The enzyme responsible for the core function of heterotrophic nitrification is pyruvic oxime dioxygenase (POD). POD is a non-heme, Fe(II)-dependent enzyme that catalyzes the dioxygenation of pyruvic oxime to produce pyruvate and nitrite. Bacteria of the genera Alcaligenes and Pseudomonas are known to perform heterotrophic nitrification, which produces nitrite from ammonia using pyruvate oxime (PO) as an intermediate metabolite. PODs have additional sequences at the N-terminus consisting of 20–30 amino acid residues that are not present in class II aldolases, corresponding to the disordered region of AfPOD in its crystal structure.

Since an AfPODdN18 variant lacking the N-terminal 18 amino acid residues showed no POD activity, the N-terminal region should play an important role in the POD activity. The crystal structures of AfPOD and AfPODdN18 were determined at resolutions of 1.76 and 1.55 Å, respectively. The structure of AfPODdN18 crystallized in the coexistence of manganese was determined as a tetramer containing 918 amino acid residues, 682 water molecules, and 4 metal ions. The N-terminal regions (Met19-Arg28) and C-terminal regions (Lys259-Arg261) of each subunit showed no apparent electron densities. The overall structure of AfPODdN18 is nearly identical to the AfPOD with a Cα root mean square deviation (RMSD) of 0.3 Å (845 Cα atoms). The anomalous difference Fourier maps suggested that the electron density near the His triad in the AfPODdN18 is not a manganese ion. Nickel or cobalt ions may have been bound to the His triad, rather than manganese, during overexpression or purification. The dN18 variant of AfPOD completely lost its enzymatic activity, indicating that the POD-specific N-terminal extension of about 30 amino acid residues, which is not present in other class II aldolases, is essential for catalytic activity.

>[4x]MATHLQQVQRDTRETMAFACRILAMTEQEAGLAGQISVRSERPGAYWTLRFGLGFDEATPEDFIEVDRDLNTLSGEGMANPATRFHLWVYEARPDVNSIIHTHSPWATVLATARQPLVISQMDMTPLHNDCAFLGEWPGVPIADQEGVIISKALGDKRAIILAHHGYLTAGKSCQEATYLSVYLERAARLQVRAQAAFGPLTPVDDTLAAEAHDYLLKPSIVNATFDYWSRQTQGIAPLTKTR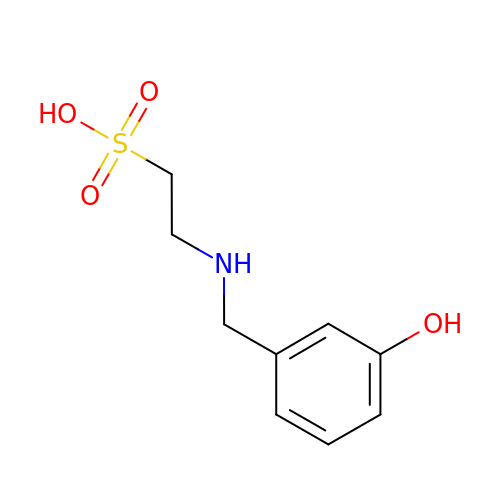2-[(3-hydroxybenzyl)amino]ethanesulfonic acid | C9 H13 N O4 S | QKFDBIPXENWQPB-UHFFFAOYSA-N2,5-BIS{[4-(N-CYCLOBUTYLDIAMINOMETHYL)PHENYL]}FURAN | C26 H32 N4 O | 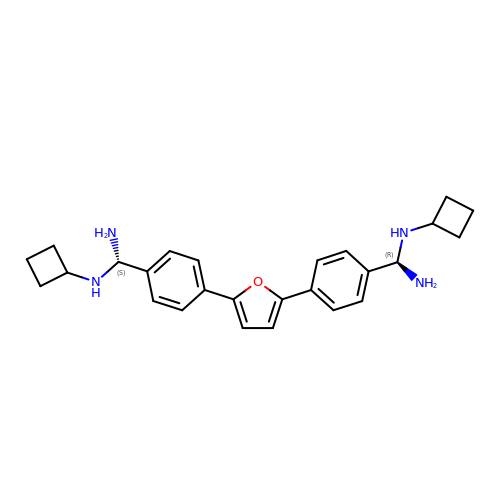PSIYSVRPSISUSW-WMPKNSHKSA-N>GPLGSMHNVLIVGASRGIGLGLADAFLQRGAQVFAVARRPQGSPGLQALAERAGERLQAVTGDLNQHDCAERIGEMLGERRIDRLIVNAGIYGPQQQDVAEIDAEQTAQLFLTNAIAPLRLARALSGRVSRGGVVAFMSSQMASLALGLSAT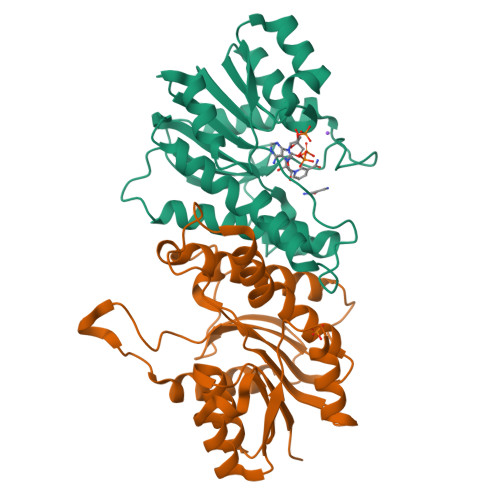MPLYGASKAALNSLVRSWEGEFEELPFSLLLLHPGWVRTEMGGDSAPLSVEESAAGLVAAVEDAAGVNACRFVDYRNQPLPW[2x]>[3x]GPSSRRAKSVEDDAEGHLIYHVG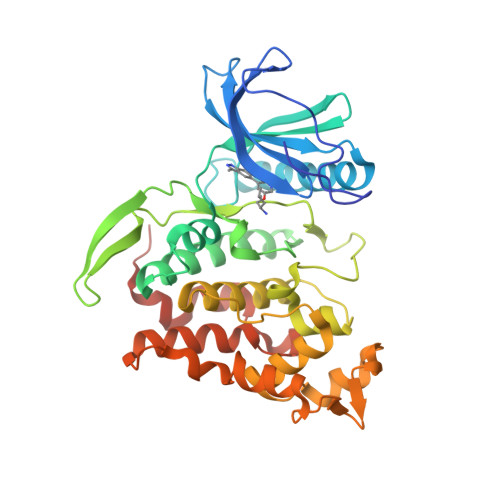DWLQERYEIVSTLGEGTFGRVVQCVDHRRGGARVALKIIKNVEKYKEAARLEINVLEKINEKDPDNKNLCVQMFDWFDYHGHMCISFELLGLSTFDFLKDNNYLPYPIHQVRHMAFQLCQAVKFLHDNKLTHTDLKPENILFVNSDYELTYNLEKKRDERSVKSTAVRVVDFGSATFDHEHHSTIVSTRHYRAPEVILELGWSQPCDVWSIGCIIFEYYVGFTLFQTHDNREHLAMMERILGPIPSRMIRKTRKQKYFYRGRLDWDENTSAGRYVRENCKPLRRYLTSEAEEHHQLFDLIESMLEYEPAKRLTLGEALQHPFFARLRAEPPNKLWDSSRD>STSAGPTVPDRDNDGIPDSLEVEGYTVDVKNKRTFLSPWISNIHEKKGLTKYKSSPEKWSTASDPYSDFEKVTGRIDKNVSPEARHPLVAAYPIVHVDMENIILSKNEDQSTQNTDSQTRTISKNTSTSRTHTSEPGSNSNSSTVAIDHSLSLAGERTWAETMGLNTADTARLNANIRYVNTGTAPIYNVLPTTSLVLGKNQTLATIKAKENQLSQILAPNNYYPSKNLAPIALNAQDDFSSTPITMNYNQFLELEKTKQLRLDTDQVYGNIATYNFENGRVRVDTGSNWSEVLPQIQETTARIIFNGKDLNLVERRIAAVNPSDPLETTKPDMTLKEALKIAFGFNEPNGNLQYQGK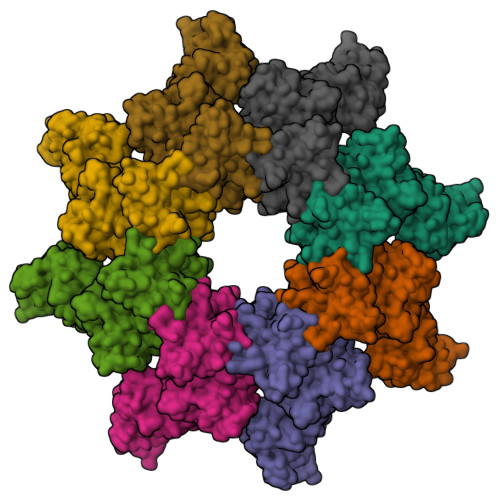DITEFDFNFDQQTSQNIKNQLAELNATNIYTVLDKIKLNAKMNILIRDKRFHYDRNNIAVGADESVVKEAHREVINSSTEGLLLNIDKDIRKILSGYIVEIEDTEGLKEVINDRYDMLNISSLRQDGKTFIDFKKYNDKLPLYISNPNYKVNVYAVTKENTIINPSENGDTSTNGIKRILIFSKKGYEIG[8x]>[2x]GAMGSEKSPSAQELKEQGNRLFVGRKYPEAAACYGRAITRNPLVAVYYTNRALCYLKMQQHEQALADCRRALELDGQSVKAHFFLGQCQLEMESYDEAIANLQRAYSLAKEQRLNFGDDIPSALRIAKKKRWNSIEERR;>[2x]XCWEAWLLCETX

Here, we report a general and rapid method for discovering α-helically constrained (Helicon) polypeptides that cooperatively induce the interaction between two target proteins without relying on previously known binders or an intrinsic affinity between the proteins. We show that Helicons are capable of binding every major class of E3 ubiquitin ligases, which are of great biological and therapeutic interest but remain largely intractable to targeting by small molecules. In addition to possessing increased stability and membrane permeability, Helicons are capable of binding large, flat protein surfaces that are inaccessible to targeting by small molecules, and Helicons have been developed to target a range of PPI targets in cells and in vivo. Characterizing Helicon-E3 co-structures and mechanisms of action, we identified new binding sites for α-helices on the E3 surfaces, as well as potential probes of the disease-linked E3, WWP123,24, highlighting the generality of our approach against this therapeutically important target class.

We performed screens of the naive phage library to identify Helicons that bind MDM2 and CHIP. Among the resulting hits, we validated CHIP-binding Helicons H317 and H318 from C80, including by x-ray crystallography to examine binding to their E3 presenters. Surprisingly, while Helicons H317 and H318 belong to the same cluster, we noted several differences in the co-structures with CHIP, reflecting unique conformational changes and binding surfaces revealed by the Helicons. For instance, the side chain of Glu9 in H317 directly interacts with Lys30 of CHIPTPR while Glu10 from H318 does not. As a proof of concept, we selected hit clusters for the RING/U-Box family E3s CHIP and MDM2, including those exemplified by H319 for MDM2 and H317 and H318 for CHIP, and designed focused libraries by fixing the conserved binding residues and diversifying the surface-exposed Helicon residues.>EDDWSKPLPPSERLEQELFSGGNTGINFEKYDDIPVEATGNNCPPHIESFSDVEMGEIIMGNIELTRYTRPTPVQKHAIPIIKEKRDLMACAQTGSGKTAAFLLPILSQIYSDGPGEALRAMKENGRYGRRKQYPISLVLAPTRELAVQIYEEARKFSYRSRVRPCVVYGGADIGQQIRDLERGCHLLVATPGRLVDMMERGKIGLDFCKYLVLDEADRMLDMGFEPQIRRIVEQDTMPPKGVRHTMMFSATFPKEIQMLARDFLDEYIFLAVGRVGSTSE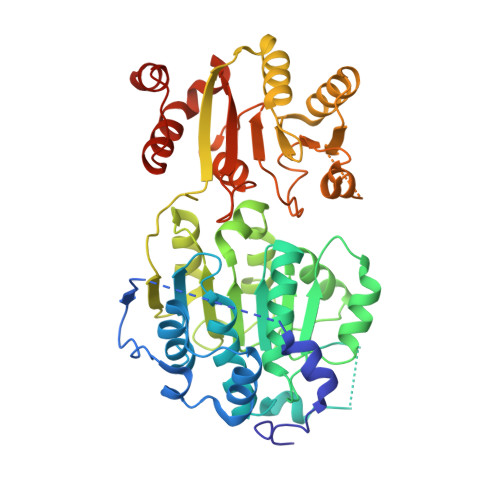NITQKVVWVEESDKRSFLLDLLNATGKDSLTLVFVETKKGADSLEDFLYHEGYACTSIHGDRSQRDREEALHQFRSGKSPILVATAVAARGLDISNVKHVINFDLPSDIEEYVHRIGRTGRVGNLGLATSFFNERNINITKDLLDLLVEAKQEVPSWLENMAYEHHYKGSS[3x]>[2x]GSAMARKRIITPEKKELIRNLISEYNITSAKDLQEALKDLLGDTIQNMLEAELDEHLGYEKYESTEEAKSNYRNGYTSKTLKSSVGQVEIDIPRDRNAEFEPKIVPRYKRDISEIENKIIAMYARGMSTREINEQIQEIYGFEVSAEMVSKITDKILPEIEEWQKRPLGEVYPIVFIDAIHFSVKNDGIVGKKAVYIVLAIDIEGQKDVIGIYVGENESSKFWLSVLNDLKNRGVKDILILCADALSGIKDAINAAFPNTEYQRCIVHQIRNTLKYVSDKDRKEFARDLKRIYTAPNEKAGYDQMLEVSEKWEKKYPAAMKSWKSNWDVICPFFKYSEELRKIMYTTNTIESLNSSYRRINKSRTVFPGDQSLLKSIYLATVKITSKWTMRYKNWGLILGQLQIMFEGRI

Copy‐out/paste‐in transposition is a major bacterial DNA mobility pathway. The pre‐reaction complex (PRC) is a complex of TnpA with DNA representing the first 26 bp of the R‐TIR with six flanking bp (fR‐TIR26); the pre‐cleaved complex (PCC) is a complex with the first 26 bp of the R‐TIR (R‐TIR26); and strand transfer complex 1 (STC1) is a complex with oligonucleotide R26(j6)L15‐5′rec in which a 6‐bp bridging spacer links two TIRs and is an approximation of the Figure‐eight intermediate. In all three complexes, a single DNA molecule is bound by a dimer of TnpA and they are all remarkably asymmetric. In each structure, the R‐TIR is recognized through an extensive protein–DNA interface in which almost all of the interactions are contributed by one protomer (“A”) with the exception of the transposon tip which is directed toward the catalytic domain (“CD”; residues 165–261 + 325–407) of the second protomer (“B”), suggesting that catalysis occurs in trans.

In the PCC, the 3′‐OH of the transferred strand (TS) points toward the active site, a position consistent with donor TIR binding rather than recipient TIR binding. The most startling difference between the protomers is that the NDB is completely disordered in one protomer (protomer B) and not detectable in the electron density. As SDS–PAGE analysis of dissolved PCC crystals indicated the presence of only full‐length TnpA, the lack of density for NDBB was not due to proteolytic degradation but rather to the spatial constraint resulting from an unusual asymmetric packing of the N‐terminal domains at the dimer interface. Although the resolution of the structures is limited and none of them contains metal ions in the active sites, in the PCC and PRC, the side chains of D175 and D241 are in the appropriate conformation for metal binding and catalysis whereas the side chain of E348 is pointing away from the presumed metal‐binding site. When we superimposed the A protomers of the PCC and PRC structures (which can be done with an overall r.m.s.d. of ~ 1.1 Å over 400 Cα positions), the clear difference is a ~ 6 Å change in the position of IDB as it closes down on the transposon end in the absence of the flanking sequence. The comparison of the active site of PCC to the active site of Hermes when bound to DNA (Hickman et al, 2018) reveals that although the 3′‐OH of the TIR end is in proximity to the catalytic residues, the scissile phosphate that would be present on the TIR end is still displaced from the equivalent position of the scissile phosphate in the Hermes complex by ~ 5 Å (assuming ideal geometry). This is likely due to a combination of factors including the lack of bound metal ion to organize the active site, stabilization of the terminal nucleotide by base pairing to the complementary strand, and the lack of flanking DNA that would be part of the authentic pre‐cleaved state.N-{2-[4-(5-chloro-2-oxo-2,3-dihydro-1H-benzimidazol-1-yl)piperidin-1-yl]ethyl}-4-fluorobenzamide 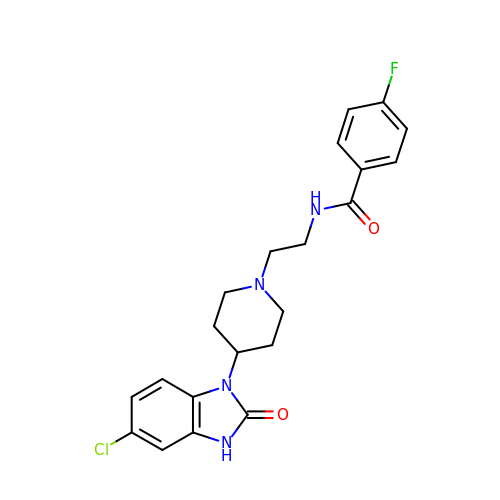| C21 H22 Cl F N4 O2 | NBHPRWLFLUBAIE-UHFFFAOYSA-N>MKPLSWSEAFGKGAGRIQASTIRELLKLTQRPGILSFAGGLPAPELFPKEEAAEAAARILREKGEVALQYSPTEGYAPLRAFVAEWIGVRPEEVLITTGSQQALDLVGKVFLDEGSPVLLEAPSYMGAIQAFRLQGPRFLTVPAGEEGPDLDALEEVLKRERPRFLYLIPSFQNPTGGLTPLPARKRLLQMVMERGLVVVEDDAYRELYFGEARLPSLFELAREAGYPGVIYLGSFSKVLSPGLRVAFAVAHPEALQKLVQAKQGADLHTPMLNQMLVHELLKEGFSERLERVRRVYREKAQAMLHALDREVP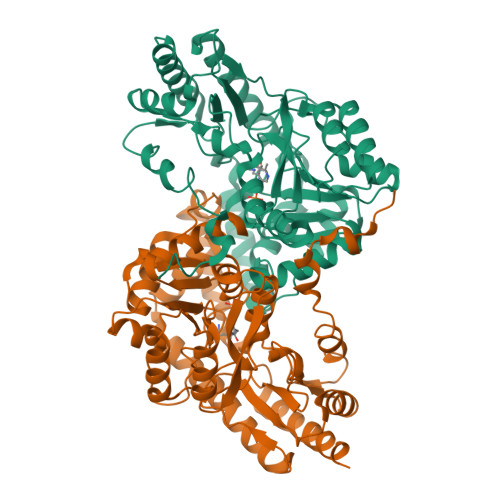KEVRYTRPKGGMFVWMELPKGLSAEGLFRRALEENVAFVPGGPFFANGGGENTLRLSYATLDREGIAEGVRRLGRALKGLLALV[4x]> ETFEIPESVTMSPKQFEGYT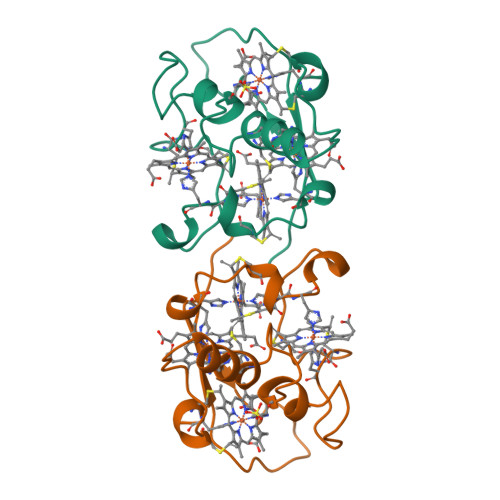PKKGDVTFNHASHMDIACQQCHHTVPDTYTIESCMTEGCHDNIKERTEISSVYRTFHTTKDSEKSCVGCHRELKRQGPSDAPLACNSCHVQ4-[2-(2-methyl-[1,2,4]triazolo[1,5-c]quinazolin-5-yl)hydrazinyl]-4-oxidanylidene-butanoic acid | 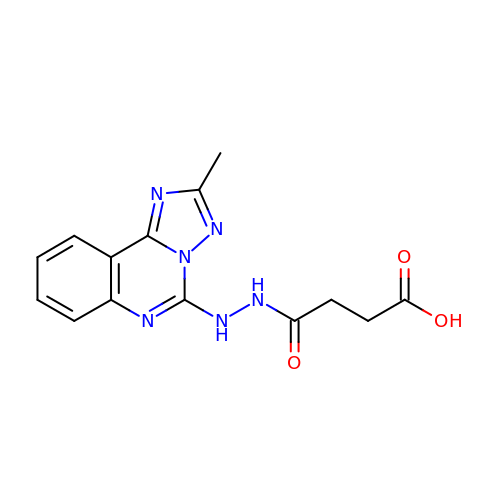C14 H14 N6 O3 | JYHOPYYRJYRCCN-UHFFFAOYSA-N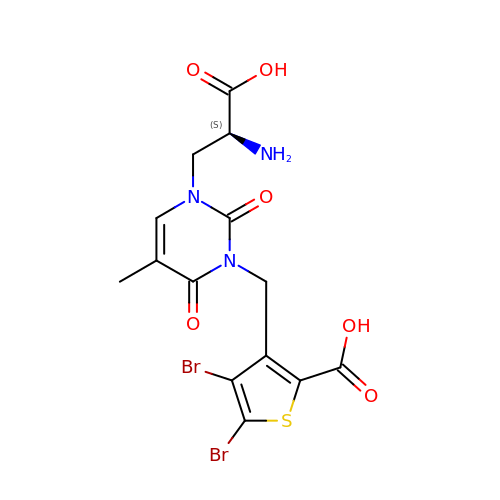3-({3-[(2S)-2-amino-2-carboxyethyl]-5-methyl-2,6-dioxo-3,6-dihydropyrimidin-1(2H)-yl}methyl)-4,5-dibromothiophene-2-carboxylic acid | C14 H13 Br2 N3 O6 S | VDFYFXPYXBDMBE-ZETCQYMHSA-N> SLLKK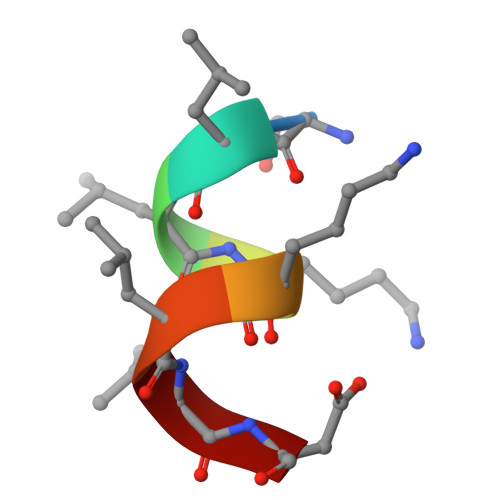LLD> MKIYGIYMDRPL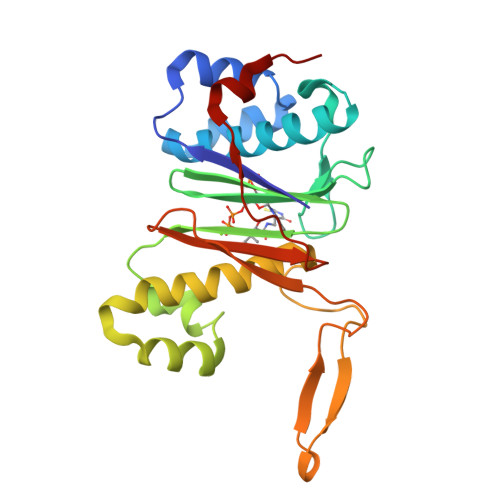SQEENERFMTFISPEKREKCRRFYHKEDAHRTLLGDVLVRSVISRQYQLDKSDIRFSTQEYGKPCIPDLPDAHFNISHSGRWVIGAFDSQPIGIDIEKTKPISLEIAKRFFSKTEYSDLLAKDKDEQTDYFYHLWSMKESFIKQEGKGLSLPLDSFSVRLHQDGQVSIELPDSHSPCYIKTYEVDPGYKMAVCAAHPDFPEDITMVSYEELLRAAA>GS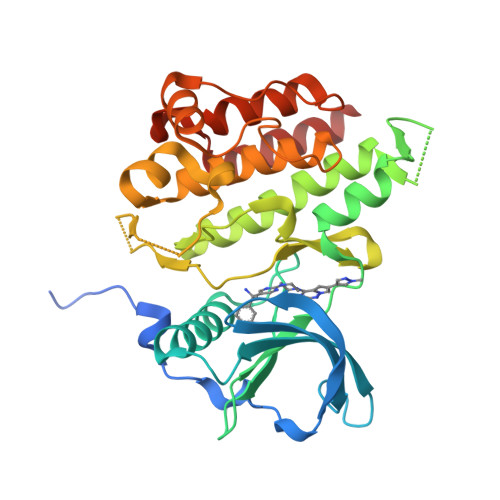MPMYEVQWKVVEESNGNNYSYIDPTQLPYDHKWEFPRNRLSFGKTLGAGAFGKVVEATAQGLIKSDAAMTVAVKMLKPSAHSTEREALMSELKVLSYLGNHENIVNLLGACTHGGPTLVIIEYCCYGDLLNFLRRKRDEFVPYKVAPEDLYKDFLTLEHLLSFSYQVAKGMAFLASKNCIHRDLAARNILLTHGNITKICDFGLARDIKNDSNYVDKGNARLPVKWMAPESIFNSVYTFESDVWSYGIFLWELFSLGSSPYPGMPVDSKFYKMIKEGFRMSSPEYAPAEMYDIMKTCWDADPDKRPTFKQIVQDIEKQISESTNH[2x]>[2x]MSTEKEKMIAGELYRSADETLSRDRLRARQLIHRYNHSLAEEHTLRQQILADLFGQVTEA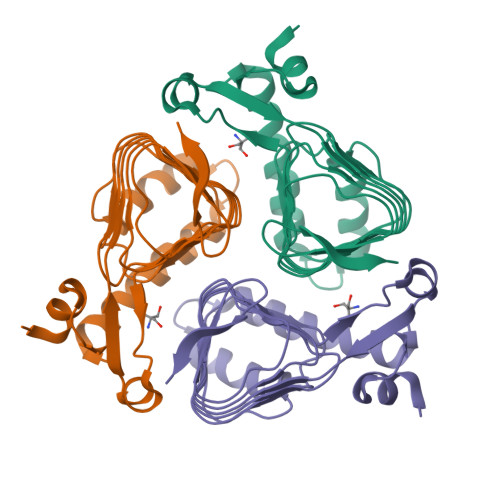YIEPTFRCDYGYNIFLGNNFFANFDCVMLDVCPIRIGDNCMLAPGVHIYTATHPIDPVARNSGAELGKPVTIGNNVWIGGRAVINPGVTIGDNVVVASGAVVTKDVPDNVVVGGNPARIIKKLLEHHHHHH> MAIASEFSSLPSYAAFATAQEAYEQAVANGDSEVVLKKLKKSLNVAKSEFDRDAAMQRKLEKMADQAMTQMYKQARSEDKRAKVTSAMQTMLFTMLRKLDNDALNNIINNARDGCVPLNIIPLTTAAK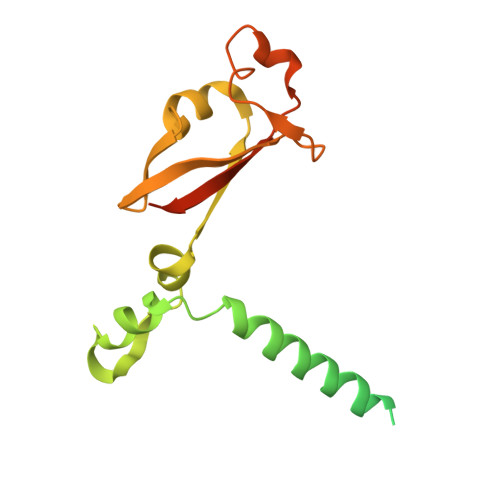LMVVIPDYNTYKNTCDGTTFTYASALWEIQQVVDADSKIVQLSEISMDNSPNLAWPLIVTALRANSAVKLQHHHHHHHH>[2x]GSMAKVEQVLSLEPQHELKFRGPFTDVVTTNLKLGNPTDRNVCFKVKTTAPRRYCVRPNSGIIDAGASINVSVMLQPFDYDPNEKSKH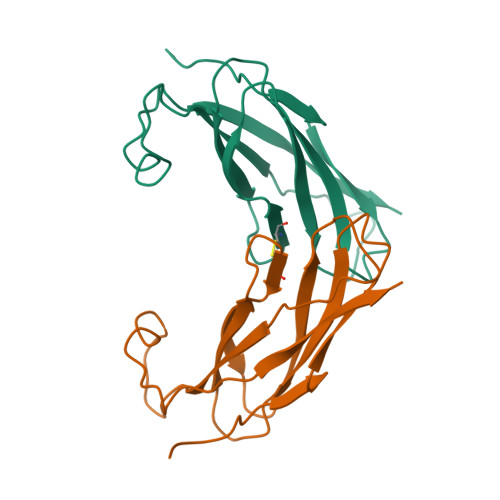KFMVQSMFAPTDTSDMEAVWKEAKPEDLMDSKLRCVFEL> MAAALRVAAVGARLSVLASGLRAAVRSLCSQATSVNERIENKRRTALLGG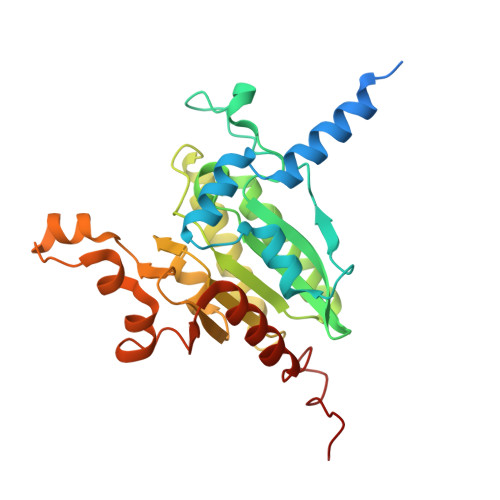GQRRIDAQHKRGKLTARERISLLLDPGSFVESDMFVEHRCADFGMAADKNKFPGDSVVTGRGRINGRLVYVFSQDFTVFGGSLSGAHAQKICKIMDQAITVGAPVIGLNDSGGARIQEGVESLAGYADIFLRNVTASGVIPQISLIMGPCAGGAVYSPALTDFTFMVKDTSYLFITGPDVVKSVTNEDVTQEELGGAKTHTTMSGVAHRAFENDVDALCNLRDFFNYLPLSSQDPAPVRECH>[24x]MLSERMLKALNDQLNRELYSAYLYFAMAAYFEDLGLEGFANWMKAQAEEEIGHALRFYNYIYDRNGRVELD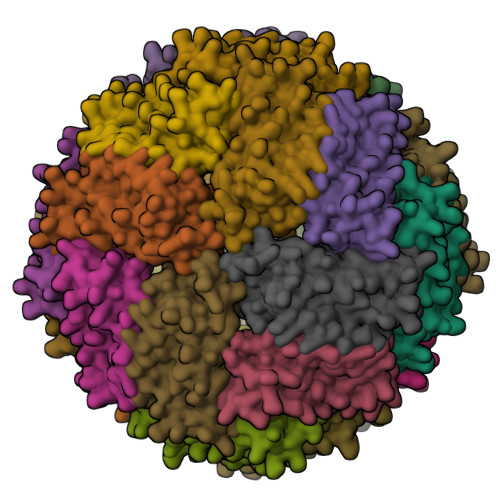EIPKPPKEWESPLKAFEAAYEHEKFISKSIYELAALAEEEKDYSTRAFLEWFINEQVEEEASVKKILDKLKFAKDSPQILFMLDKELSARAPKLPGLLMQGG> MAV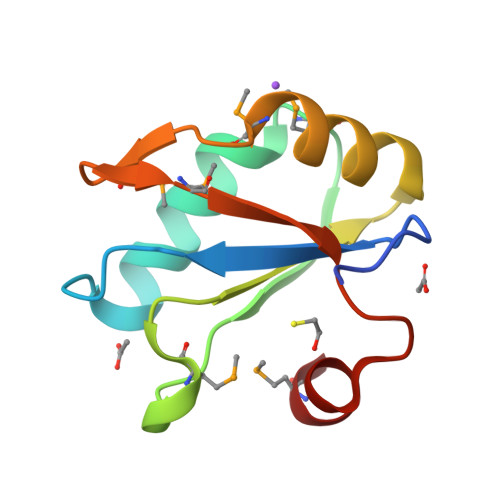PETRPNHTIYINNLNEKIKKDELKKSLHAIFSRMGQILDILVSRSLKMRGQAFVIFKEVSSATNALRSMQGFPMYDKPMRIQYAKTDSDIIAKMK>GPGFDFAQAIMKKNTVIARTEKGEFTMLGVYDRVAVIPTHASVGETIYINDVETKVLDACALRDLTDTNLEITIVKLDRNQKFRDIRHFLPRYEDDYNDAVLSVHTSKFPNMYIPVGQVTNYGFLNLGGTPTHRILMYNFPTRAGQAGGVVTTTGKVIGIHVGGNGAQGFAAMLLHSYFSDTQ[2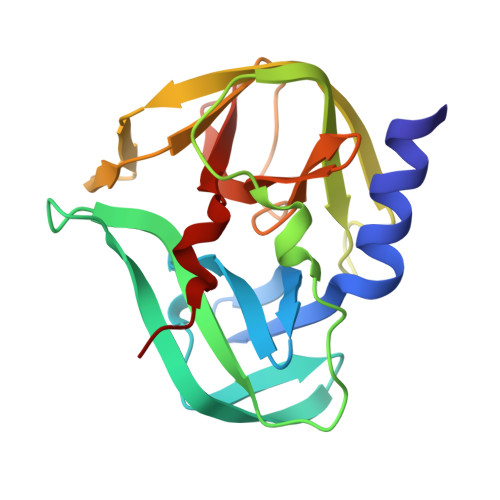x]> MTMPLRGLGPPDDTGVREVSTGDDHHY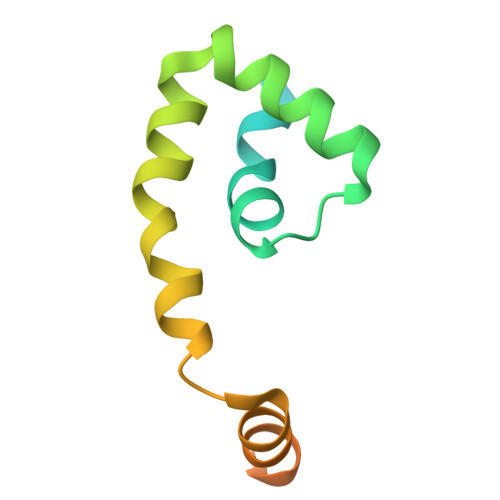AMWDAAYVLGALSAADRREFEAHLAGCPECRGAVTELCGVPALLSQLDRDEVAAISESAPTVVASGLSPELLPSLLAAVHR>GGGGGAGGGGTACAGGGGTACAG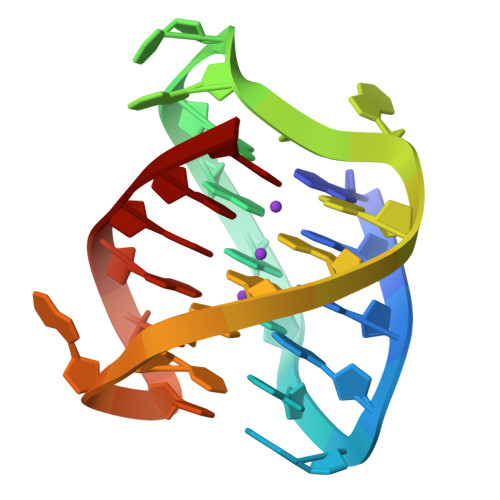GGG[7x]> MNVDNVKSQMRKGMLEYCIMLLLHK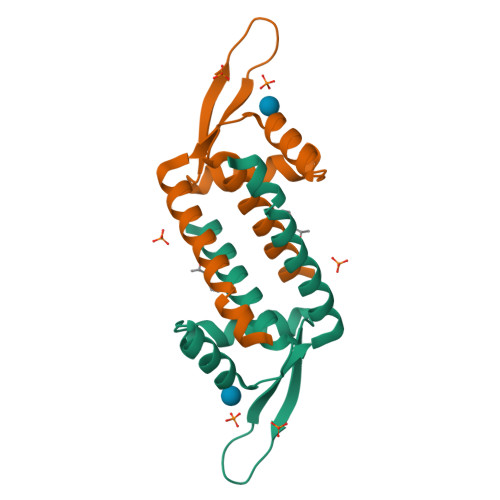EPAYASDIIQKLKEARLIVVEGTLYPLLTRLKNDDLLSYEWVESTQGPPRKYYKLTGKGESFLGELEASWKELNETVNHIANRESI>[2x]EQARPADDALAALGAQLFVDPALSRNATQSCATCHDPARAFTDPREGKAGLAVSVGDDGQSHGDRNTPTLGYAALVPAFHRDANGKYKGGQFWDGRADDLKQQAGQPMLNPVEMAMPDRAAVAARLRDDPAYRTGFEALFGKGVLDDPERAFDAAAEALAAYQATGEFSPFDSKYDRVMRGEEKFTPLEEFGYTVFITFNCRLCHMQRKQGVAERETFTNFEYHNIGLPVNETAREASGLGADHVDHGLLARPGIEDPAQSGRFKVPSLRNVAVTGPYMHNGVFTDLRTAILFYNKYTSRRPEAKINPETGAPWGEPEVARNLSLAELQSGLMLDDGRVDALVAFLETLTDRRYEPLLEESRAAQKDHHHHHH;>ADAPAGTDPRAKWVPQDNDIQACDYWRHCSIDGNICDCSGGSLTNCP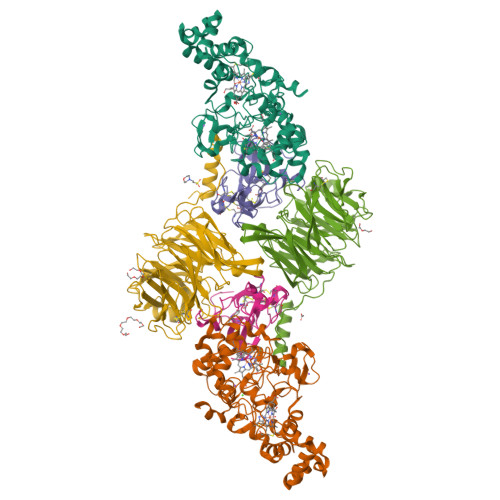PGTKLATASWVASCYNPTDGQSYLIAYRDCCGYNVSGRCPCLNTEGELPVYRPEFANDIIWCFGAEDDAMTYHCTISPIVGKASHHHHHH[2x];>[2x]QDAPEAETQAQETQGQAAARAAAADLAAGQDDEPRILEAPAPDARRVYVNDPAHFAAVTQQFVIDGEAGRVIGMIDGGFLPNPVVADDGSFIAHASTVFSRIARGERTDYVEVFDPVTLLPTADIELPDAPRFLVGTYPWMTSLTPDGKTLLFYQFSPAPAVGVVDLEGKAFKRMLDVPDCYHIFPTAPDTFFMHCRDGSLAKVAFGTEGTPEITHTEVFHPEDEFLINHPAYSQKAGRLVWPTYTGKIHQIDLSSGDAKFLPAVEALTEAERADGWRPGGWQQVAYHRALDRIYLLVDQRDEWRHKTASRFVVVLDAKTGERLAKFEMGHEIDSINVSQDEKPLLYALSTGDKTLYIHDAESGEELRSVNQLGHGPQVITTADMG> MTMITHHHHHHGSTSITDFLRLTGNEFASVAQDGVTAGDISGWVDSGSYAFNALLSGDIYKGFPGNKIVVIGADPSTGKTFFALGAAKNFLEQNKDGIVICFESESAITKNMLVERGIDVKRFGVVPVSTVQQFKTQALRIVDNYEKQPKNERQPVLFILDSLGMLSTDKEMADSAEGKDTRDMTRAQLIKAAFRVLTLKLGRAGIPMIVTNHVYEDVGAGPYASKVQAGGSGAVYASSTILTLSKAKDRDTSTNEVTGVIVTVTATKSRLTKENSKIKCLIRYDGGLDRYYGMLELAEEAGVFKKVSTRFELEDGTKLFGKTIMENPEKYFTNDILERI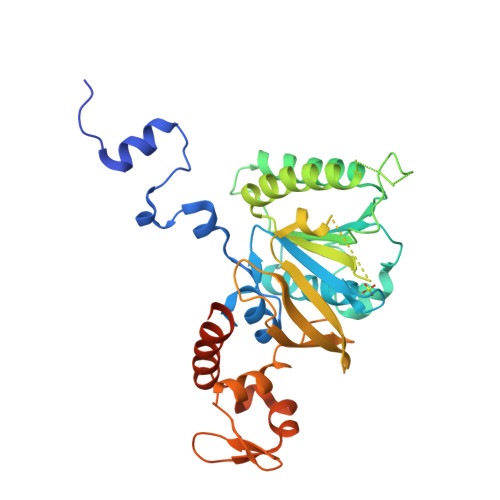NDYVKRKFCYGSGDDQAGADETLDDDEGQGDIH>[2x]MSLAADSADAGFARDMSVHHQQAVEMSYIVRDRTDDEEVRRLAYDIAQTQANQRGMMIGWLDLWALPKVSSDPPMTWMGMGDAPSAGEGSLMPGMATDAEMKKLGTLDG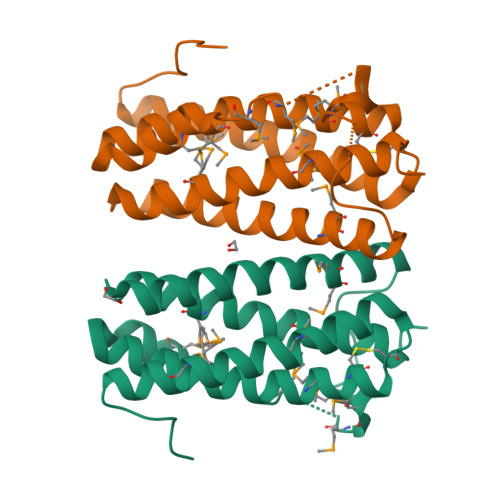KQAEVYYLQLMTEHHRGGVHMAKGCVERCTVGVEKRLARGMVESQESEIRLMADLLAERGAKEGHHHHHH>[6x]MDEAVGDLKQALPCVAESPTVHVEVHQRGSSTAKKEDINLSVRKLLNRHNIVFGDYTWTEFDEPFLTRNVQSVSIIDTELKVKDSQPIDLSACTVALHIFQLNEDGPSSENLEEETENIIAANHWVLPAAEFHGLWDSLVYDVEVKSHLLDYVMTTLLFSDKNVNSNLITWNRVVLLHGPPGTGKTSLCKALAQKLTIRLSSRYRYGQLIEINSHSLFSKWFSESGKLVTKMFQKIQDLIDDKDALVFVLIDQVESLTAARNACRAGTEPSDAIRVVNAVLTQIDQIKRHSNVVILTTSNITEKIDVAFVDRADIKQYIGPPSAAAIFKIYLSCLEELMKCQIIYPRQQLLTLRELEMIGFIENNVSKLSLLLNDISRKSEGLSGRVLRKLPFLAHALYVQAPTVTIEGFLQALSLAVDKQFEERKKLAAYI;> MAAPEAEVLSSAAVPDLEWYEKSEETHASQIELLETSSTQEPLNASEAFCPRDCMVPVVFPGPVSQEGCCQFTCELLKHIMYQRQQLPLPYEQLKHFYRKPSPQAEEMLKKKPRATTEVSSRKCQQALAELESVLSHLEDFFARTLVPRVLILLGGNALSPKEFYELDLSLLAPYSVDQSLSTAACLRRLFRAIFMADAFSELQAPPLMGTVVMAQGHRNCGEDWFRPKLNYRVPSRGHKLT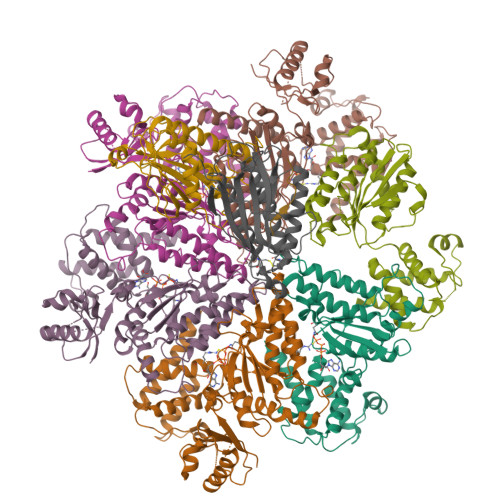VTLSCGRPSIRTTAWEDYIWFQAPVTFKGFRE;> MAQFAFESDLHSLLQLDAPIPNAPPARWQRKAKEAAGPAPSPMRAANRSHSAGRTPGRTPGKSSSKVQTTPSKPGGDRYIPHRSAAQMEVASFLLSKENQPENSQTPTKKEHQKAWALNLNGFDVEEAKILRLSGKPQNAPEGYQNRLKVLYSQKATPGSSRKTCRYIPSLPDRILDAPEIRNDYYLNLVDWSSGNVLAVALDNSVYLWSASSGDILQLLQMEQPGEYISSVAWIKEGNYLAVGTSSAEVQLWDVQQQKRLRNMTSHSARVGSLSWNSYILSSGSRSGHIHHHDVRVAEHHVATLSGHSQEVCGLRWAPDGRHLASGGNDNLVNVWPSAPGEGGWVPLQTFTQHQGAVKAVAWCPWQSNVLATGGGTSDRHIRIWNVCSGACLSAVDAHSQVCSILWSPHYKELISGHGFAQNQLVIWKYPTMAKVAELKGHTSRVLSLTMSPDGATVASAAADETLRLWRCFELDPARRREREKASAAKSSLIHQGIR;> MALQLSREQGITLRGSAEIVAEFFSFGINSILYQRGIYPSETFTRVQKYGLTLLVTTDLELIKYLNNVVEQLKDWLYKCSVQKLVVVISNIESGEVLERWQFDIECDKTAKDDSAPREKSQKAIQDEIRSVIRQITATVTFLPLLEVSCSFDLLIYTDKDLVVPEKWEESGPQFITNSEEVRLRSFTTTIHKVNSMVAYKIPVND> MGFIDLLKPAFSLIPEVQPARQYIPKDHKIVWTGITLFIYLVCCQIPLYGVVRAQGSDPFYWMRVILASNRGTLMELGISPLVTSSMIVQLLVNTRILDFNARVQDDRQAIQGAQKLLGLIMSMCEAFAYIWSGQYGDPNKIGLGSCLLIFIQLVFSGIVVLLLDDMLNKGYGLGSGISLFIATNICENIVWRSFSPITITTQQGTEFE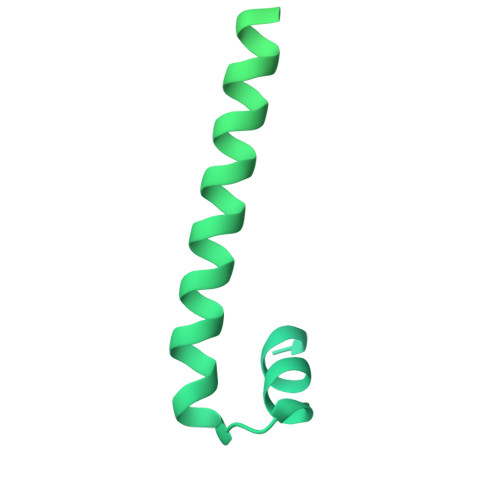GSIINLFHSLLTKDRVSNALYHSFYRTSAPNLVNLISTLLVFLVVIYLQGVKYDLRIARRQERNSESSYPIKLFYTSNYPIILQTALVSQIFFFSRILSSKFKNNFFVKLLGQWQDGSVAGGQDHPIGGFVYFLTAPRDLNQVISDPIHAIFYVLIILTLCGVISRYWIEFSDESTSSVHKKFMEEKIEIPGHRQDSVYRTLDRIIPTAATLGGICVGVLTIVADFLGAIGSGTGILLAVNIIYGYFEQVKKENKLKKTGIVQQQQQQM> GHMERLLDELTLEGVARYMQSERCRRVICLVGAGISTSAGIPDFRSPSTGLYDNLEKYHLPYPEAIFEISYFKKHP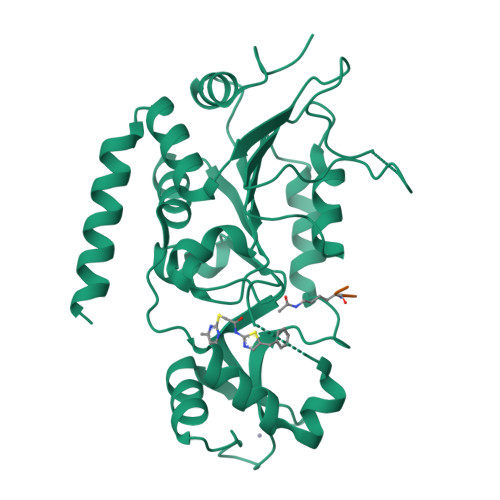EPFFALAKELYPGQFKPTICHYFMRLLKDKGLLLRCYTQNIDTLERIAGLEQEDLVEAHGTFYTSHCVSASCRHEYPLSWMKEKIFSEVTPKCEDCQSLVKPDIVFFGESLPARFFSCMQSDFLKVDLLLVMGTSLQVQPFASLISKAPLSTPRLLINKEKAGQSDPFLGMIMGLGGGMDFDSKKAYRDVAWLGECDQGCLALAELLGWKKELEDLVRREHASIDAQS;> EKR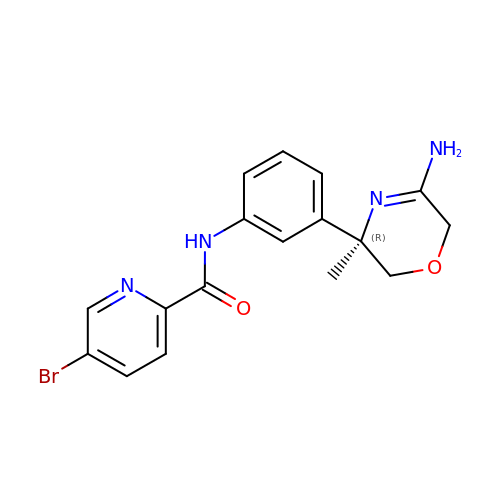~{N}-[3-[(3~{R})-5-azanyl-3-methyl-2,6-dihydro-1,4-oxazin-3-yl]phenyl]-5-bromanyl-pyridine-2-carboxamide | C17 H17 Br N4 O2 | HALWMQVNBCAXRZ-KRWDZBQOSA-N> RLMTRIALDPFVRDLDGESAALRAAGPLAEVELPGGVHVYAVTHHKEARALLTDSRVVKDINVWNAW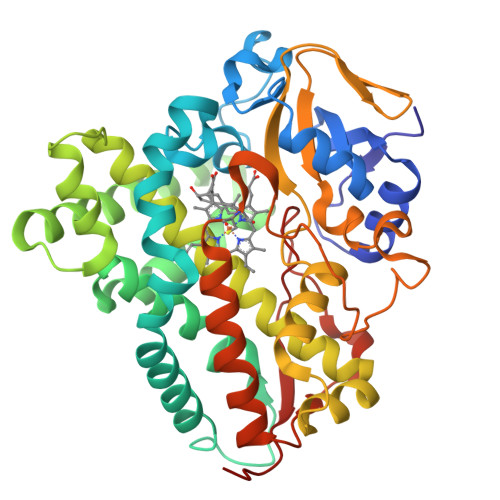QRGEIPADWPLIGLVNPGRSMLTVDGPDHRRLRTLVAQALTVKRVEKLRAGIEALTNASLERLAALPAGEPVDLKAEFAYPLPMNVISELMGVDAADHPRLKELFEKFFSTQTPPEEVPQMMADLGTLFTKIVEEKKANPGDDLTSALIAASEDGDHLTDEEILNTLQLIIAAGHETTISLIVNVVEALAIHPEQRKKVLSGEIPWEGVIEETLRWNTPTSHVLIRFATEDIEVGDKVLPKGEGLVVSFGALGRDEEQYGPTAGDFDATRTPNRHIAFGHGPHVCPGAALSRLEAGIALPALYERFPELDLAVPAAELRNKPIVTQNDLHDLPVKLGCPFGHDA>[2x]MAHHHHHHMFTLSTDPHASKAELYATLAEQARSLVESEPDLIANAANFSALVYHSLDRLNWAGFYFFDGTELVVGPFQGKPACVRIALGKGVCGTAAQTRQTQVVRD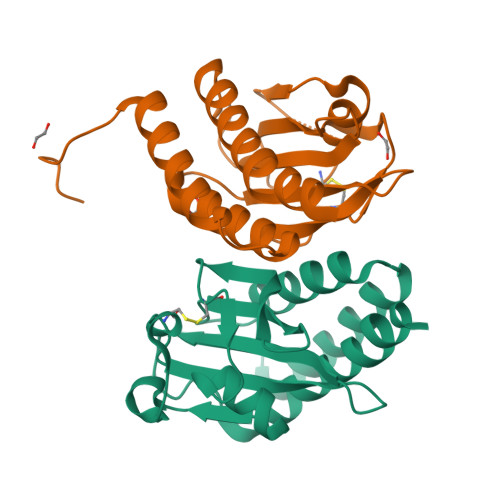VHAFPGHIACDAASESEIVVPLVAADGTLIGVWDVDSPVAARFDDEDRSGMEALCRVFVEHAWQKARDRAA> SMSDLHIPGTQSTPAIQGDWQAGRLSMQGDSYPENSYELFGQVIDWVERFLADGQRPLELDLRLL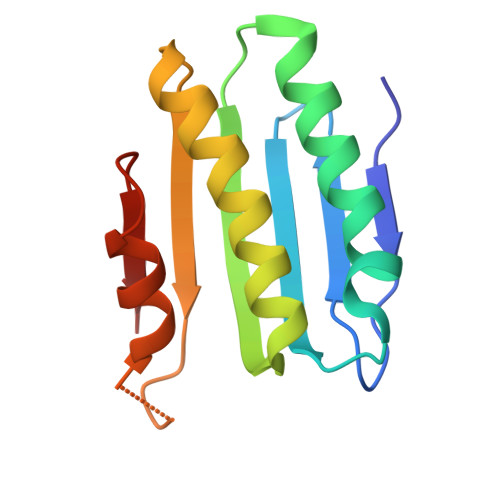YLNTSSIKAMMDILDLLEEAHQGGRPVSLRWHYDRRNERVAELAEEFREDCSFPFAIQAHDE> MNTIAWLGRLVIERIRGIGVAALMLLQIIFSLPSAGGFGRFVYQMHRVGVMSLLIITVSGLFIGLVLGLQGYSILVNVGSESMLGTMVSLTLLRELAPVVAALLFAGRAGSALTAEIGSMKQSEQLAS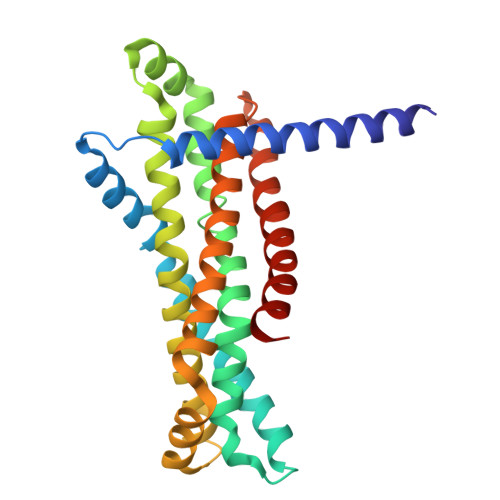MEMIGVDPLKQIVSPRLWAGIVSLPMLTVIFAAIGIVGGKLVGVDFLGVDEGSFWSGMQNNVQFGHDVVNGIIKSIVFALLCTWIAVFQGYACDPTPEGIATAMTRTVVYSSLCVLGFDFVLTAVMFGGI3-((9,9-dimethyl-9H-fluoren-2-yl)methyl)-2-oxoglutarate | C21 H20 O5 | 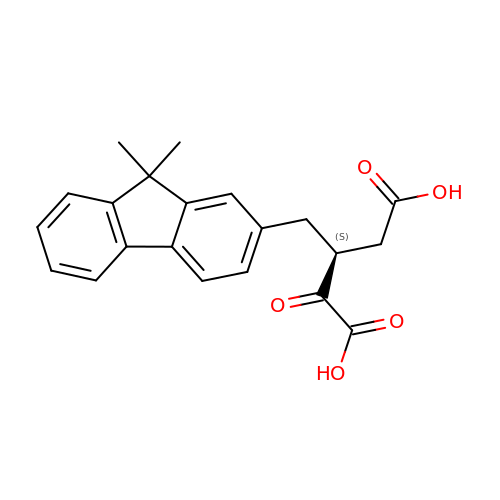VBQHCGIHMLAMOB-ZDUSSCGKSA-N Protoglobin (Pgb) is a recently discovered haem-protein with distinct structural and functional features that make it unique within the globin superfamily. The MaPgb* structure can be considered as an expanded version of the 3/3 helical sandwich typical of “classical” globins (i.e. Mb), with an additional N-terminal extension, built by a 20-residue loop, followed by the Z-helix, which precedes the globin-fold conserved A-helix. Residues belonging to the Z-helix contribute to formation of the Pgb homodimer, which is centered on the intermolecular four-helix bundle built by the G- and H-helices of the two subunits. Thus, in Pgb the access of diatomic ligands, such as O2, CO, and NO, to the haem is granted by two orthogonal apolar tunnels that reach the haem distal region from entry sites at the B/G and B/E helix interfaces.

The Tyr(61)B10Ala mutation has instead a dramatic impact on the accessibility of the haem distal site since it increases the average tunnel 2 diameter by more than 1.5 Å (6.0 Å is the shortest distance between Ala(61)B10 Cβ atom and the surrounding residues). As a result of such increased accessibility, the tunnel 2 entrance site (i.e. roughly the cavity left by the Tyr→Ala mutation) in the Tyr(61)B10Ala mutant hosts a glycerol molecule (in both chains A and B; the glycerol molecule bound to chain A is modeled in a double conformation) which is able to H-bond the haem-Fe(III)-bound cyanide (distance of ∼2.8–2.9 Å, depending on the protein chain). Thus, in the Tyr(61)B10Ala mutant, the haem-Fe(III)-bound cyanide molecule is stabilized by the interaction with the Trp(60)B9 Nε2 atom (2.92 Å for chain A, and 2.90 Å for chain B), and by the additional H-bond provided by the glycerol molecule which mimics the H-bond provided by the Tyr(61)B10 OH group in the MaPgb*(III)-cyanide structure. As a result, both the orientations of the haem-Fe(III)-bound cyanide molecule and of the Phe(93)E11 side chain match those found in the MaPgb*(III)-cyanide structure. Furthermore, the presence of the Trp(60)B9 side chain within the haem distal site affects the orientation of the haem-Fe(III)-bound cyanide, but does not impact on the ability of the adjacent Tyr(61)B10 residue to reorient its side chain toward the haem-Fe(III)-bound-ligand, as demonstrated by the structure of the cyanide-bound Trp(60)B9Ala mutant. Similarly, the Tyr(61)B10Ala mutation does neither impair the Phe(93)E11 ligand-sensing mechanism described above, nor ligand stabilization provided by Trp(60)B9. Higher accessibility to the haem-distal ligand-binding site due to the Tyr(61)B10Ala and Trp(60)B9Ala mutations may also partly contribute for the increase in koff for cyanide. off for cyanide dissociation from Trp(60)B9Ala MaPgb*(III)-cyanide and Tyr(61)B10Ala MaPgb*(III)-cyanide species are closely similar to those reported for cyanide dissociation from Mb(III)-cyanide and Hb(III)-cyanide complexes, where ligand stabilization is achieved through the distal HisE7 residue.

>MSVEKIPGYTYGETENRAPFNLEDLKLLKEAVMFTAEDEEYIQKAGEVLEDQVEEILDTWAGFVGSHPHLLYYFTSPDGTPNEKYLAAVRKRFSRWILDTSNRSYDQAWLDYQYEIGLRHHRTKKNQTDNVESVPNIGYRYLVAFIYPITATMKPFLARKGHTPEEVEKMYQAWFKATTLQVALWSYPYVKYGDF[2x]> MTNRTPRISAIRSAALAALLAGLGMGAAQATEFRSADTHNADDYPTVAAVKYMGELLEKKSGGKHKIKVFNKQALGSEKETIDQVKIGALDFTRVNVGPMNAICPLTQVPTMPFLFSSIAHMRKSLDGPVGDEILKSCESAGFIGLAFYDSGARSIYAKKPIRTVADAKGLKIRVQQSDLWVALVSAMGANATPMPYGEVYTGLKTGLIDAAENNIPSFDTAKHVEAVKVYSKTEHSMAPEILVMSKIIYDKLPKAEQDMIRAAAKESVAFERQKWDEQEAKSLANVKAAGAEIVEVDKKSFQAVMGPVYDKFM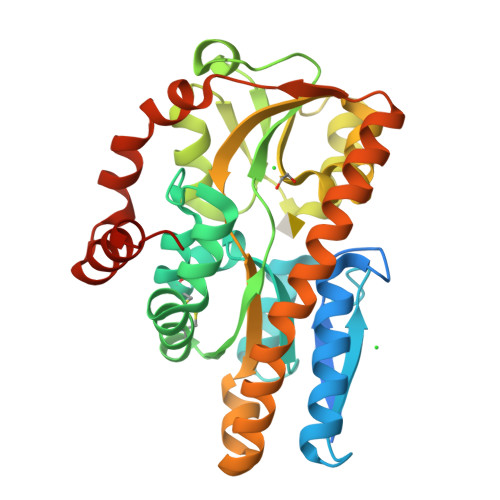TTPDMKRLVKAVQDTKAENLYFG>GPGSCPTHADSLNNLANIKREQGNIEEAVRLYRKALEVFPEFAAAHSN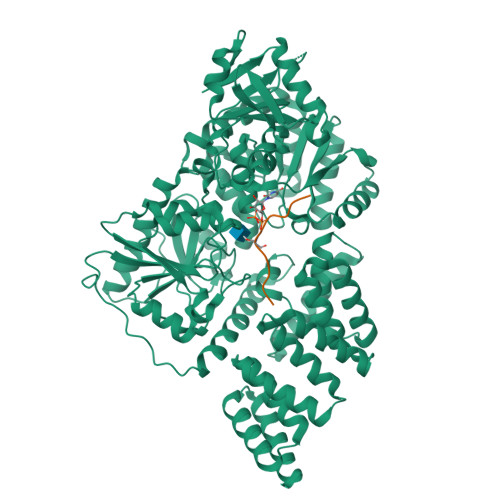LASVLQQQGKLQEALMHYKEAIRISPTFADAYSNMGNTLKEMQDVQGALQCYTRAIQINPAFADAHSNLASIHKDSGNIPEAIASYRTALKLKPDFPDAYCNLAHCLQIVCDWTDYDERMKKLVSIVADQLEKNRLPSVHPHHSMLYPLSHGFRKAIAERHGNLCLDKINVLHKPPYEHPKDLKLSDGRLRVGYVSSDFGNHPTSHLMQSIPGMHNPDKFEVFCYALSPDDGTNFRVKVMAEANHFIDLSQIPCNGKAADRIHQDGIHILVNMNGYTKGARNELFALRPAPIQAMWLGYPGTSGALFMDYIITDQETSPAEVAEQYSEKLAYMPHTFFIGDHANMFPHLKKKAVIDFKSNGHIYDNRIVLNGIDLKAFLDSLPDVKIVKMKCPDGGDNADSSNTALNMPVIPMNTIAEAVIEMINRGQIQITINGFSISNGLATTQINNKAATGEEVPRTIIVTTRSQYGLPEDAIVYCNFNQLYKIDPSTLQMWANILKRVPNSVLWLLRFPAVGEPNIQQYAQNMGLPQNRIIFSPVAPKEEHVRRGQLADVCLDTPLCNGHTTGMDVLWAGTPMVTMPGETLASRVAASQLTCLGCLELIAKNRQEYEDIAVKLGTDLEYLKKVRGKVWKQRISSPLFNTKQYTMELERLYLQMWEHYAAGNKPDHMIKPVE[4x];>[4x]PVSVPYSSAQS>CCGAAUGAG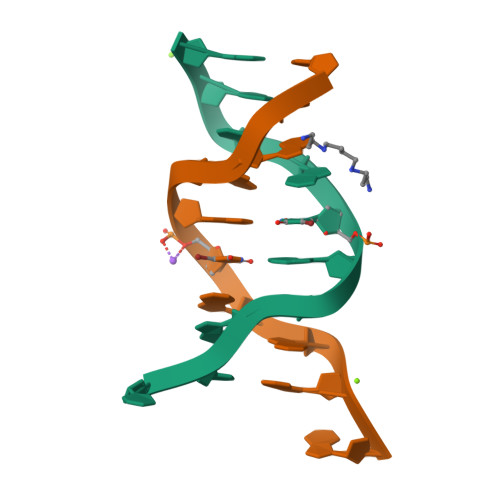G[2x]> MKNPEEAADGKQRIHLRPGSLRGAAPAKLHLLPCDVLVSRPAPVDRFFTPAVRHDADGLQASFRGRGLRGEEVAVPPGFAGFVMVTEEKGEGLIGKLNFSGDAEDKADEAQEPLERDFDRLIGATGSFSHFTLWGLETVPGPDAKV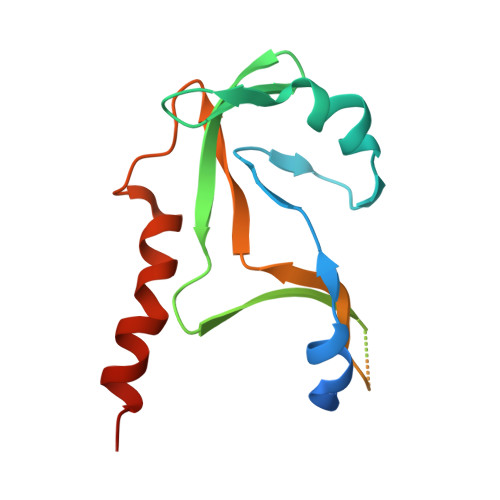HRALGWPSLAAAIHAQVPED>MDSSRFSGNKSTYTDLQTTSEQFLFSSESVCSGHPDKLCDQISDAILDACLEQDPESFVACETCTKTGFIMVFGEITTKANVNYERVVRETVKEIGYDSEEKGLDYKTMDVIIKLEQQSNQIAGCVHVDKNVEDIGAGDQGMMFGYATNETKELMPLTHVLATSITRELDYIRVKGVSSRVGWLRPDGKAQVTVEYNCKHGVLIPKRIHTILVSVQHDENIENEEIREFVLENVIKKVCPSDLMDKETRILINPSGRFTIGGPAADAGLTGRKIIVDTYGGWGAHGGGAFSGKDATKVDRSGAYMARLVAKSIV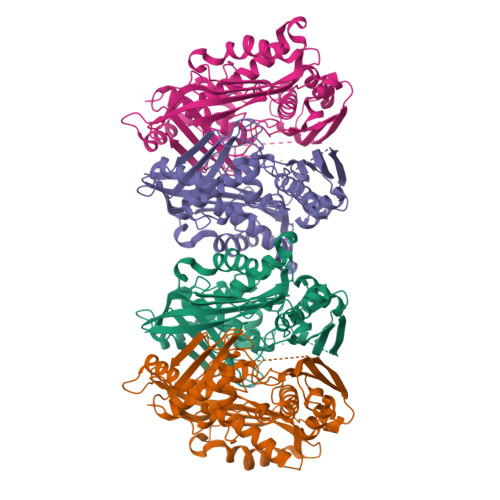FSGLCSRCLVQVSYGIGIARPLSLYINTFGTAKDGYNDAKLLEIVNKVFDFRPGILIKQLNLKSPIFKKTSSGGHFGRSEEEFLWEKPIILQ[4x]>[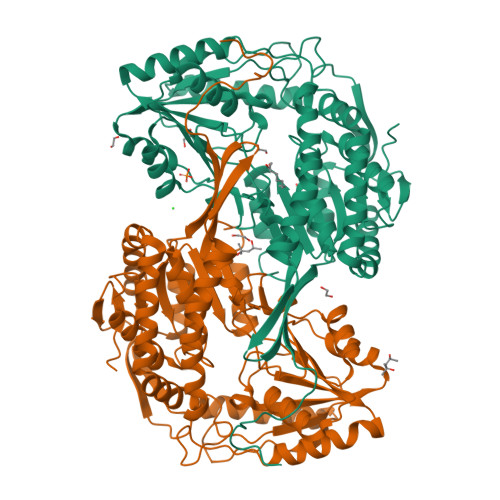2x]MHHHHHHANLTGNVYIDGLWLPGHGAPFESVQPVTGETVWDGNAASLEDVDAAVREARKAFLAWRRKSLAERQAVIEAFGELLEANKEELAHQIGLETGKPLWESRTEVAAMMGKIPISVKAYNERTGHTESDVAGGHAVLRHRPHGVVAVFGPYNFPGHLPNGHIVPALLAGNTVVFKPSELTPGVAELTVRLWEKAGLPDGVINLVQGGSDTGKCLARHSLIDGLFFTGSSTVGHLLHEQFGGQPEKILALEMGGNNPLIVQNVSDLDGAVHHALQSAFLSAGQRCTCARRLLVPKGKKGDEFLARLVEVAARITVAEFDADPQPFMGSVISAEAANQLLKAQAAMLEKGATSLLEMKQLKPDTGLLSPGIVDATGIELEDQEFFGPLLTVYRYKGFDEALELANNTRYGLSAGILSDDRKLYNRLVEEVRAGIVNWNRPLTGASSAAPFGGVGASGNHRPSAYYAADYCAWPMASLEAGKSELPDSLAPGLNFD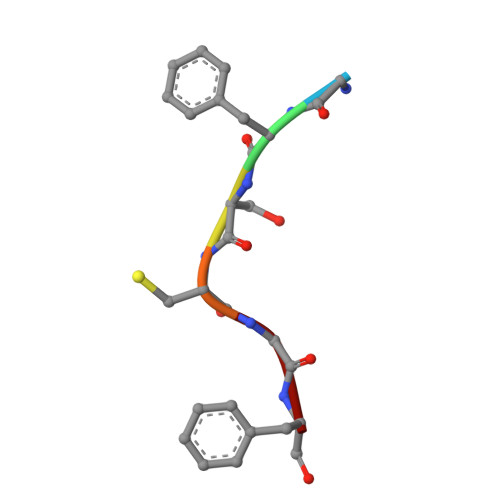> GFSCGF>MDLTERQRKVLLFIEEFIEKNGYPPSVREIARRFRITPRGALLHLIALEKKGYIERKNGKPRALRISKSIRNKIPLIGEIRAGEKREAIEYLEDYIEIPESFLSSGYDHFLLKVKGESMIEEHICDGDLVLVRRQDWAQNGDIVAAMVDGEVTLAKFYQRGDTVELR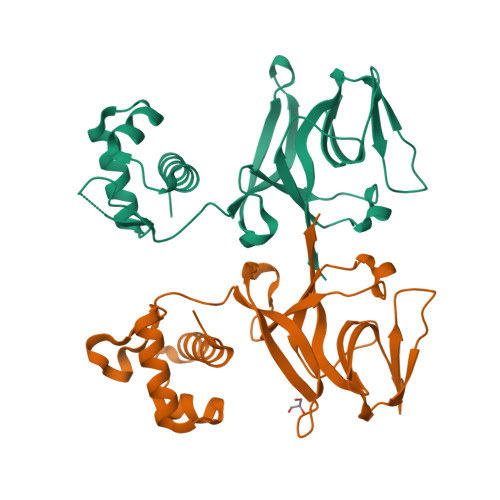PANREMSSMFFRAEKVKILGKVVGVFRKL[2x]2-[5-[1,1,2,2-tetrakis(fluoranyl)ethyl]-1~{H}-pyrazol-3-yl]phenol 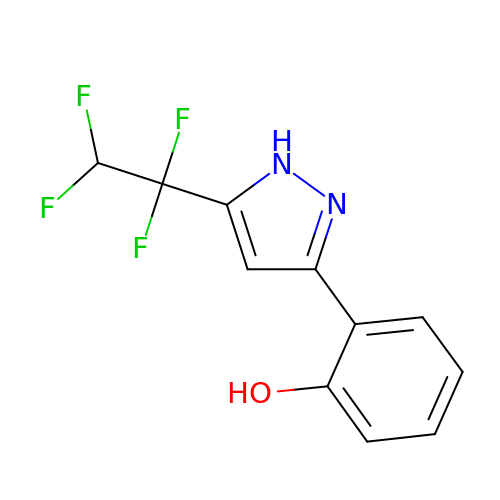| C11 H8 F4 N2 O | AZBWBPKELVSJMM-UHFFFAOYSA-N>MAEFRIAQDVVARENDRRASALKEDYEALGANLARRGVDIEAVTAKVEKFFVAVPSWGVGTGGTRFARFPGTGEPRGIFDKLDDCAVIQQLTRATPNVSLHIPWDKADPKELKARGDALGLGFDAMNSNTFSDAPGQAHSYKYGSLSHTNAATRAQAVEHNLECIEIGKAIGSKALTVWIGDGSNFPGQSNFTRAFERYLSAMAEIYKGLPDDWKLFSEHKMYEPAFYSTVVQDWGTNYLIAQTLGPKAQCLVDLGHHAPNTNIEMIVARLIQFGKLGGFHFNDSKYGDDDLDAGAIEPYRLFLVFNELVDAEARGVKGFHPAHMINQSHNVTDPIESLINSANEIRRAYAQALLVDRAALSGYQEDNDALMATETLKRAYRTDVEPILAEAR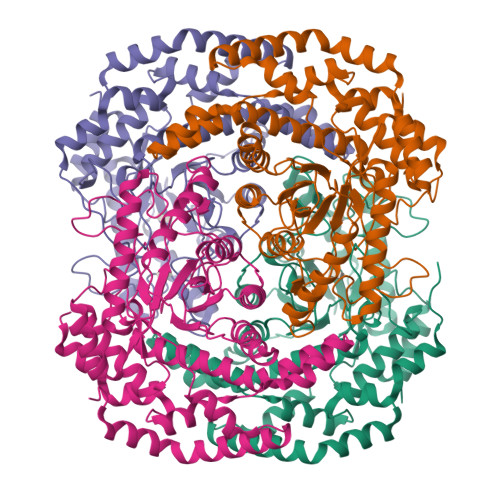RRTGGAVDPVATYRASGYRARVAAERPASVAGGGGIIGSHHHHHH[4x]>LALMSAAKLPKSFVWGYATAAYQIEGSPDKDGREPSIWDTFCKAPGKIADGSSGDVATDSYNRWREDVQLLKSYGVKAYRFSLSWSRIIPKGGRSDPVNGAGIKHYRTLIEELVKEGITPFVTLYHWDLPQALDDRYGGWLNKEEAIQDFTNYAKLCFESFGDLVQNWITFNEPWVISVMGYGNGIFAPGHVSNTEPWIVSHHIILAHAHAVKLYRDEFKEKQGGQIGITLDSHWLIPYDDTDASKEATLRAMEFKLGRFANPIYKGEYPPRIKKILGDRLPEFTPEEIELVKGSSDFFGLNTYTTHLVQDGGSDELAGFVKTGHTRADGTQLGTQSDMGWLQTYGPGFRWLLNYLWKAYDKPVYVTENGFPVKGENDLPVEQAVDDTDRQAYYRDYTEALLQAVTEDGADVRGYFGWSLLDNFEWAEGYKVRFGVTHVDYETQKRTPKKSAEF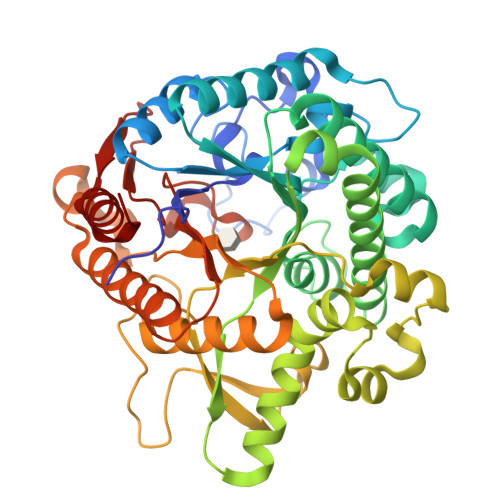LSRWFKEHIEE[2x]>MADDQGCIEEQGVEDSANEDSVDAKPDRSSFVPSLFSKKKKNVTMRSIKTTRDRVPTYQYNMNFEKLGKCIIINNKNFDKVTGMGVRNGTDKDAEALFKCFRSLGFDVIVYNDCSCAKMQDLLKKASEEDHTNAACFACILLSHGEENVIYGKDGVTPIKDLTAHFRGDRCKTLLEKPKLFFIQACRGTELDDGIQAD[2x];>SGPINDTDANPRYKIPVEADFLFAYSTVPGY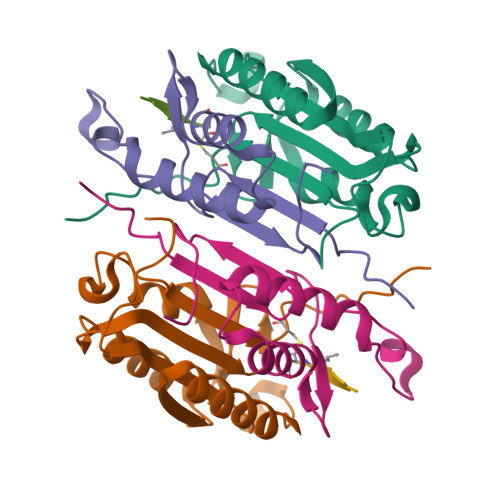ASMRNPGRGSWFVQALCSILEEHGKDLEIMQILTRVNDRVARHFESQSDDPHFHEKKQIPCVVSMLTKELYFSQLEHHHHHH[2x]> MKLALAALLATSAAAFQAPTMTFSLGKKAAAKKAVKAPAPSGASPSADAWANSIESKALPFARAPATLDGTMLGDFGFDPLGFSTVPVGPWFTGIEGRNGQIGNLNWYREAELIHGRIAQVAVVGFIAP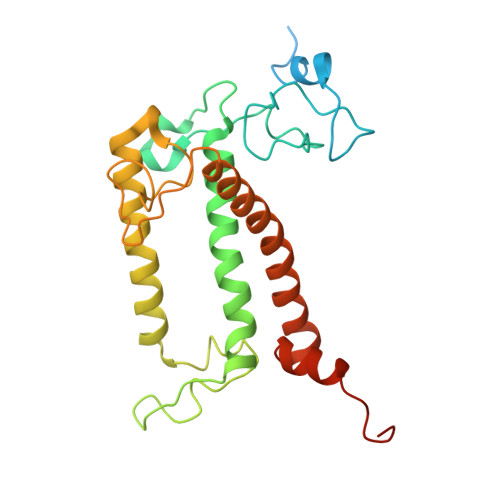GLFGTLPGNEWTGVDAYSNLNPLEAFSQVPGLAILQIFLFMSYLEVRRINIIKEEGENYMPGDLRIGQGEGRWNPFGLDYSPEAYEEKRLQELKHCRLAMIGVFGLWAQAQASGVGVTEQIGAALTTPDYYAKAGYFLPEGI> MLITREQLMKIASIPLKRKEPEYNLILDALENFNRDIEGTSVKEIYSKLSKLNELVDNYQTKYPSSGRNLALENFRDSLYSELRELIKNSRTSTIASKNLSFIWIGGPISDQSLEYYNMWKMFNKDYNIRLFYDKNSLLVNTLKTAIIQESSKVIIEQNQSNILDGTYGHNKFYSDRMKLIYRYKRELKMLYENMKQNNSVDDIIINFLSNYFKYDIGKLNNQKENNNNKMIAIGATDINTENILTNKLKSYYYQELIQTNNLAAASDILRIAILKKYGGVYCDLDFLPGVNLSLFNDISKPNGMDSNYWEAAIFEAIANEKKLMNNYPYKYMEQVPSEIKERILSFVRNHDINDLILPLGDIKISQLEILLSR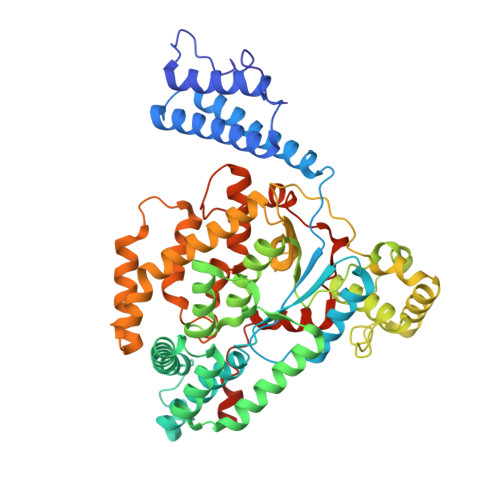LKAATGKKTFSNAFIISNNDSLTLNNLISQLENRYEILNSIIQEKFKICETYDSYINSVSELVLETTPKNLSMDGSSFYQQIIGYLSSGFKPEVNSTVFFSGPNIYSSATCDTYHFIKNTFDMLSSQNQEIFEASNNLYFSKTHDEFKSSWLLRSNIAEKEFQKLIKTYIGRTLNYE>[7x]MAENTKNENITNILTQKLIDTRTVLIYGEINQELAEDVSKQLLLLESISN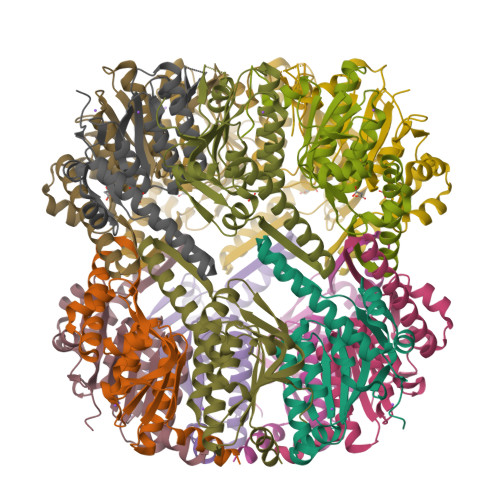DPITIFINSQGGHVEAGDTIHDMIKFIKPTVKVVGTGWVASAGITIYLAAEKENRFSLPNTRYMIHQPAGGVQGQSTEIEIEAKEIIRMRERINRLIAEATGQSYEQISKDTDRNFWLSVNEAKDYGIVNEIIENRDGLKMASWSHPQFEK;>MNLIPTVIEQTSRGERAYDIYSRLLKDRIIMLGSAIDDNVANSIVSQLLFLDAQDPEKDIFLYINSPGGSISAGMAIYDTMNFVKADVQTIGMGMAASMGSFLLTAGANGKRFALPNAEIMIHQPLGGAQGQATEIEIAARHILKIKERMNTIMAEKTGQPYEVIARDTDRDNFMTAQEAKDYGLIDDIIINKSGLKGHHHHHH[7x]> GSHMKNSVSVDLPGSMKVLVSKSSNADGKYDLIATVDALELSGTSDKNNGSGVLEGVKADASKVKLTISDDLGQTTLEVFKSDGSTLVYKYVYSKDKSYTYEYFNEKGEVSYKYIYRADG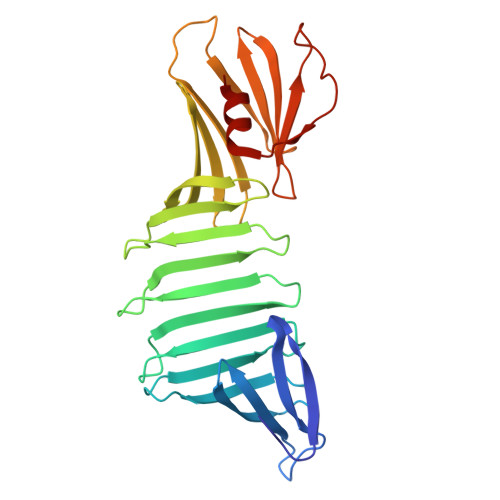TRLEYTGIKSDGSGKAKEVLKGYVLEGTLTAEKTTLVVKEGTVTLSKNISKSGEVSVELNDTDSSAATKKTAAWNSGTSTLTITVNSKKTKDLVFTSSNTITVQQYDSNGTSLEGSAVEITKLDEIKNALK> MELIKGQALFLELDKKDFLSLKNNDKNIPTFAHPKNQEKILAIFSLPYKNPPQNTKLIAFYKDKKEEIFIKTLEGNYKSEKLQVENKKIFPPKTIQERIAKELKEANAIYSSYTPKALFNGAFNIPLNSFITSDFGKARTFNEKVASYHSGTDFRAATGTPIYAANSGVVKIAKDRYFAGNSVVIDHGFGIYSQYYHLSKIDVKVGQKIKKGELIGLSGASGRVSGPA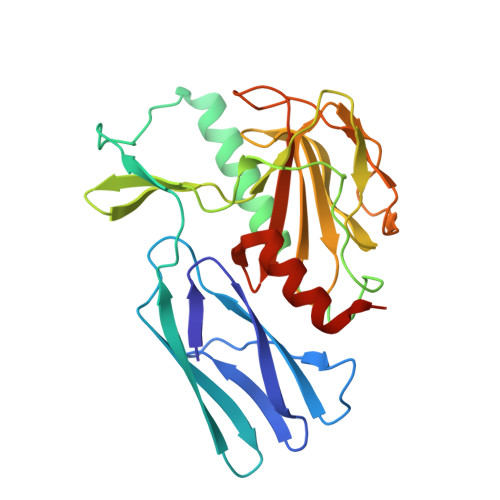LHFGILAGGKQVDPLDFVSKFNAIFQLEHHHHHH> ANSFLEEVKQGNLERECLEEACSLEEAREVFEDAEQTDEFWSK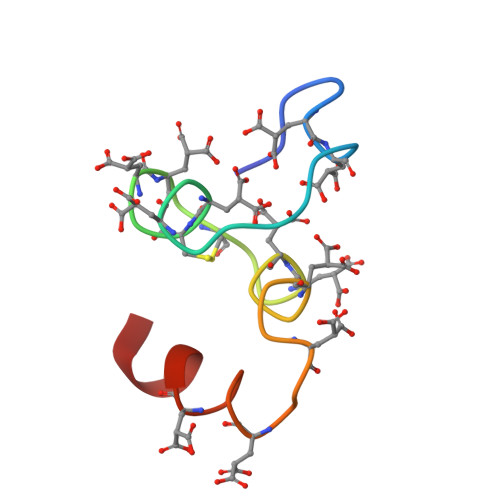Y> TGGTHTPKLKHLDKLLAHCHRRRYTAKSTIIYAGDRCETLFFIIKGSVTILIEDDDGREMIIGYLNSGDFFGELGLFEKEGSEQERSAWVRAKVECEVAEISYAKFRELSQQDSEILYTLGSQMADRLRKTTRKVGDLAFLDVTGRVARTLLDLCQQPDAMTHPDGMQIKITRNEIGRIVGCSREMVG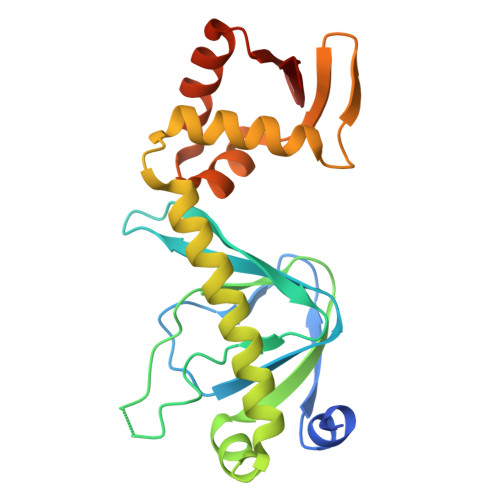RVLKSLEEQGLVHVKGKTMVVFGTR In some cases, when there is a short upstream open reading frame (uORF) that precedes the main ORF, ribosomes can translate the uORF, terminate translation, and then undergo a poorly understood process called “translation reinitiation” whereby they resume scanning for another AUG initiation codon and then translate the main ORF. We previously showed that two noncanonical initiation factors, density-regulated reinitiation and release factor (DENR) and multiple copies in T-cell lymphoma-1 (MCTS1), are involved in this process. The structure of MCTS1 contains a pseudouridine synthase and archaeosine transglycosylase (PUA) domain fold typically present in proteins that bind RNA. DENR contains an SUI1 domain, similar to eukaryotic initiation factor 1 (eIF1).

Instead, we assembled and crystallized the minimal complex consisting of full-length wild-type (WT) MCTS1 and residues 24–51 of DENR and determined its crystal structure to 2.14-Å resolution. Although we initially determined the structure by molecular replacement, strong positive density near MCTS1-His58 and the three Cys residues of DENR suggested the presence of a metal ion, most likely zinc. We therefore collected a dataset at the Zn-edge and could determine the structure de novo by means of Zn–single-wavelength anomalous dispersion (SAD). The overall structure of MCTS1 is essentially the same as the previously reported crystallization variant MCTS1x, as indicated by the low root-mean-square deviation (RMSD) of 0.71 Å for 181 residues. The DENR N-terminus (residues 25 to 33) is largely extended, lacking secondary structure, while the C-terminal part contains a partial zinc finger (residues 34 to 44) and a short α-helix (residues 44 to 46), which, according to secondary structure prediction, would extend to residue 60. The N-terminus of DENR (residues 25–33) is unfolded and crawls along the N-terminal domain of unknown function 1947 of MCTS1. The majority of residues involved in DENR binding are conserved—in particular, Leu82, Leu170, and Trp175, which form a hydrophobic surface. An extensive network of hydrogen bonds is formed between DENR-Glu42 and the backbones of MCTS1-Gln140 and His141, between DENR-Tyr43 and MCTS1-Lys139, between DENR-Tyr43 and the carbonyl of MCTS-His141, and between DENR-Tyr46 and MCTS1-Lys139. Our structure now reveals that Cys37 is part of this zinc finger. From our structure of MCTS1–DENR(aa24–51), Phe104 of MCTS1 is predicted to stack against the last base in the acceptor stem of tRNA, thereby “measuring” the length of the tRNA and allowing RNAs that terminate at that position to bind efficiently.

> MFKKFDEKENVSNCIQLKTSVIKGIKNQLIEQFPGIEPWLNQIMPKKDPVKIVRCHEHIEILTVNGELLFFRQREGPFYPTLRLLHKYPFILPHQQVDKGAIKFVLSGANIMCPGLTSPGAKLYPAAVDTIVAIMAEGKQHALCVGVMKMSAEDIEKVNKGIGIENIHYLNDGLWHMKTYK;> MHHHHHHDADYPLRVLYCGVCSLPTEYCEYMPDVA> GSHMEKTGLHVHEKIKHMVKNYGTMITGIPAEILGQNEAEISVGYVKKMGNMKENIAEVVRKSEMTQPTNSAGKASNEVCDLLLGTEGASEFEKSSYQVLSGDGSNLKGSLPNKNLLVRVEMDRFNAPQKYQKIKREEFNPETAEKNKIYLLEDQLVYLDIFGKVIDLGQTSDTCHRLFNAITTPFYQNYILYDEYIDPEESAEEAAMFEMGEIVKAKMKNIDCWTATHSFTIFVPESDSEDTRTLYPYQAYWTSHTLQQWFSGDKDEKLSRLGIDGYIEKLALLGTTTDSKIRSSIYGELFSPPGKEHVFCTGMNEKFSPLRVKFKVTEVNPEIALQNLEEVQEFIDTNYPGENAKDQCELYKIKAQEAMTKQLEMRLLIE;> GSHMFFKDYQKKNVMRLLQDSLEKIINEWLKTDDESHTKLKSLQELSEMDINATSFAEHSPLPDFVTRLWLDPHKALDAMDKNISKNEIRKLIKETAREIELVFTHQK

Recently, two L. pneumophila effectors MavC and MvcA, were identified as structural homologs of cycle inhibiting factor (Cif) effectors. MavC catalyzes the transglutamination reaction between Ub and UBE2N, leading to UBE2N ubiquitination in an unconventional form. Non-canonical ubiquitination of UBE2N by MavC abolishes its activity in the formation of K63-type polyubiquitin chains, which dampens NF-κB signaling in the initial phase of L. pneumophila infection. Here, we report the structures of the MavC/UBE2N/Ub ternary complex, MavC/UBE2N–Ub (product) binary complex, and MavC/Lpg2149 binary complex, which provide important insights into the mechanism and inhibition of this transglutaminase-induced ubiquitination by MavC.

To investigate the inhibition mechanism of Lpg2149, we reconstituted the MavC–Lpg2149 complex in vitro and solved its crystal structure. The complex structure revealed that MavC and Lpg2149 bind as a 1:1 dimer, consistent with the molecular weight of the complex measured by gel filtration coupled with static light scattering (SLS) analyses. Lpg2149 has an overlapped binding site with Ub in MavC, but does not interfere with UBE2N binding, indicating that Lpg2149 inhibits the activity of MavC through competing with Ub to bind MavC. Lpg2149 extensively interacts with MavC via multiple contact points, burying a surface area of 2229 Å2. Lpg2149 interacts with both the head and tail region of the main domain of MavC mainly through two contacting regions, namely contact A3 and B3. Contact A3, involving the N-terminal long α1 helix (residues 11–38) of Lpg2149, contains six pairs of hydrogen bonds: the sidechain nitrogen of Lpg2149Q16 with the main-chain carbonyl oxygen of MavCG30, the amide nitrogen of Lpg2149F12 with the sidechain of MavCE344, the sidechain hydroxyl of Lpg2149S27 with the sidechain of MavCN39, the sidechain hydroxyl of Lpg2149Y15 with the main-chain carbonyl oxygen of MavCI28, and the sidechain of Lpg2149N19 with the main-chain carbonyl oxygen of MavCT29. Moreover, hydrophobic interactions between F11/F12 of Lpg2149 and N341/F348 of MavC, and between V20/L23/L24 of Lpg2149 and I31/I35/N39 of MavC further anchor the complex conformation. In contact B3 which involves the α3/α4 helix region (residues 70–77/79–82) of Lpg2149, the sidechain of MavCQ38 forms two hydrogen bonds with the sidechain oxygen of Lpg2149D84 and the amide nitrogen of Lpg2149A85. Lpg2149 F11A/F12A, F11K/F12D, Y15A/K18A/N19A, and V20A/L23A/L24A mutations, designed to disrupt MavC–Lpg2149 interaction, all showed decreased MavC binding as detected both by isothermal titration calorimetry (ITC) assay and IC50 analysis. Superimposition of the MavC molecules in the MavC/Lpg2149 and MavC/UBE2N–Ub complexes also shows a rotation of around 6° of the helical-bundle tail region, where both Lpg2149 and Ub bind, indicating a binding-induced movement of the helical-bundle tail region.> NEYAPLRLHVPEPTGRPGCQTDFSYLRLNDAGQARKPPVDVDAADTADLSYSLVR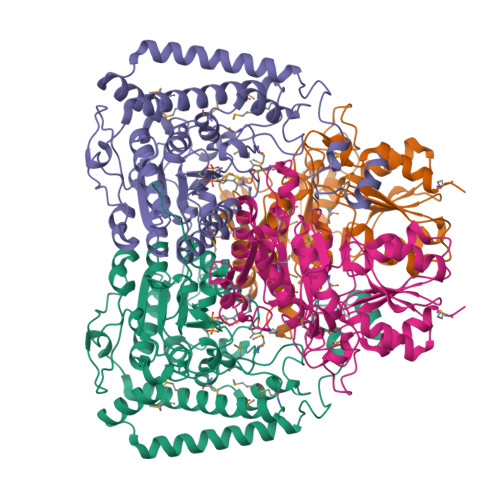VLDEQGDAQGPWAEDIDPQILRQGMRAMLKTRIFDSRMVVAQRQKKMSFYMQSLGEEAIGSGQALALNRTDMCFPTYRQQSILMARDVSLVEMICQLLSNERDPLKGRQLPIMYSVREAGFFTISGNLATQFVQAVGWAMASAIKGDTKIASAWIGDGATAESDFHTALTFAHVYRAPVILNVVNNQWAISTFQAIAGGESTTFAGRGVGCGIASLRVDGNDFVAVYAASRWAAERARRGLGPSLIEWVTYRAGPHSTSDDPSKYRPADDWSHFPLGDPIARLKQHLIKIGHWSEEEHQATTAEFEAAVIAAQKEAEQYGTLANGHIPSAASMFEDVYKEMPDHLRRQRQEL;> ATTTMTMIQALRSAMDVMLERDDNVVVYGQDVGYFGGVFRCTEGLQTKYGKSRVFDAPISESGIVGTAVGMGAYGLRPVVEIQFADYFYPASDQIVSEMARLRYRSAGEFIAPLTLRMPCGGGIYGGQTHSQSPEAMFTQVCGLRTVMPSNPYDAKGLLIASIECDDPVIFLEPKRLYNGPFDGHHDRPVTPWSKHPHSAVPDGYYTVPLDKAAITRPGNDVSVLTYGTTVYVAQVAAEESGVDAEVIDLRSLWPLDLDTIVESVKKTGRCVVVHEATRTCGFGAELVSLVQEHCFHHLEAPIERVTGWDTPYPHAQEWAYFPGPSRVGAALKKVMEV> MTVVSAFLVPGTPLPQLKPEVPSWGQLAAATERAGKALAASRPDVVLVYSTQWL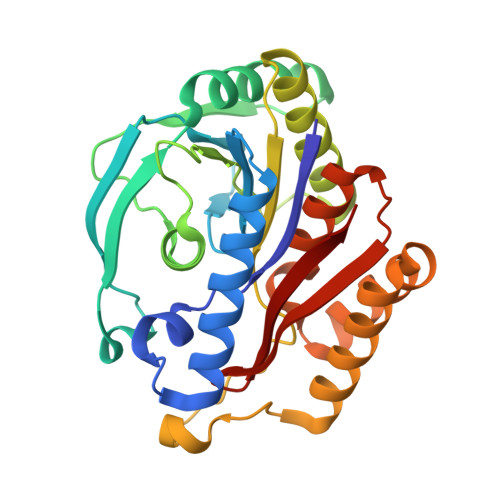AVLDQQWLTRPRSEGVHVDENWYEFGDLAYDIRADTALAEACVTSSPLHGVHARGVNYDGFPIDTGTITACTLMGIGTDAFPLVVGSNNLYHSGEITEKLAALAVDCAKDQNKRVAVVGVGGLSGSLFREEIDPREDRIANEEDDKWNRRVLKLIEAGDVSALREAMPVYAKEARVDMGFKHLHWILGALKGKFSGANVLGYGPSYGSGAAVIEFRL> MHHHHHHSLLTEVETYVLSIVPSGPLKAEIAQRLEDVFAGKNTDLEVLMEWLKTRPILSPLTKGILGFVFTLTVPSERGLQRRRFVQNALNGNRDPNNMDKAVK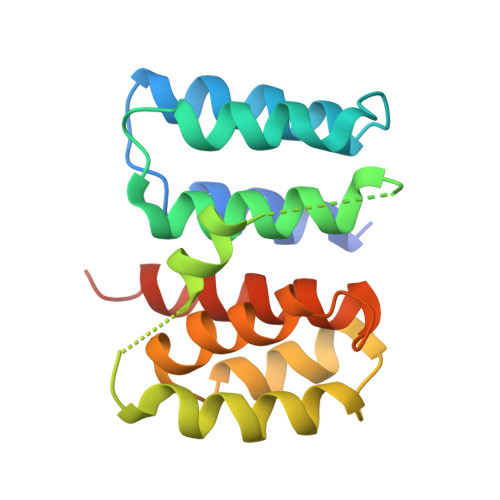LYSKLKSEITFHGAKEIALSYSAGALASCMGLIYNRMGAVTTEVAFGLVCATCEQIADSQHRSHRQM> GSEEVVQDAPLENNELNAE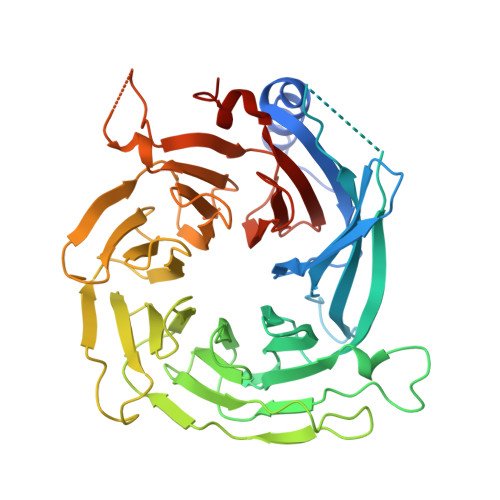IDLQKTIQEEYKLWKQNVPFLYDLVITHALEWPSLTIQWLPDKKTIPGTDYSIQRLILGTHTSGNDQNYLQIASVQLPNFDEDTTEFTPSTIRRAQATGSYTIEISQKIPHDGDVNRARYMPQKPEIIATMGEGGNAYIFDTTCHDALTTGEALPQAVLKGHTAEGFGLCWNPNLPGNLATGAEDQVICLWDVQTQSFTSSETKVISPIAKYHRHTDIVNDVQFHPQHEALLASVSDDCTLQIHDTRLNPEEEAPKVIQAHSKAINAVAINPFNDYLLATASADKTVALWDLRNPYQRLHTLEGHEDEVYGLEWSPHDEPILASSSTDRRVCIWDLEKIGEEQTPEDAEDGSPELLFMHGGHTNRISEFSWCPNERWVVGSLADDNILQIWSPSRVIWGRDHVQVSPRDLE2'-DEOXYCYTIDINE-2'-DEOXYADENOSINE-3',5'-MONOPHOSPHATE | C19 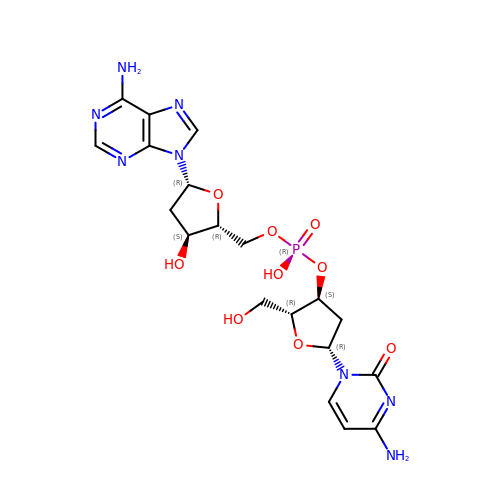H25 N8 O9 P | LYWWDKIADIGKTH-IDMWBNCISA-N> MIEKLIHFINNDLLEGAADDLDQNTPLLELGILDSLSMVLLLAHIDQQYGVKIPEHEINPEHFENVATLAALINQLS;> MNFEWTHEQAELFEHALRFGKELSAPLQEDNGFPRDNWNALGDFGYFGLPIPEKYAKDGSGFDILTTIKIIEGLGQSCTDTGLLFAGAAHTFACSMPILEHGSETLKHQLLPDLATGRKIAANAISEASAGSDISNLATTAQKEGDYYVLNGGKSYVTNGSIADYYVVYATTNKKHGYLGQTAFVVPRNTPGISVGNDYHKLGLRSAPLNQVFFDNCTIHKDYALGREGQGARIFAASMDWERCCLFAIFVGAMQRDLNQCIEYANTRMQGDKTISRFQAVSHRIADMGVRLESARLMLYYAAWQKSQDVDNTKAVAMSKLAISEAFVQSGIDSIRVHGALGYLDEGRVNNSIKDALGSVL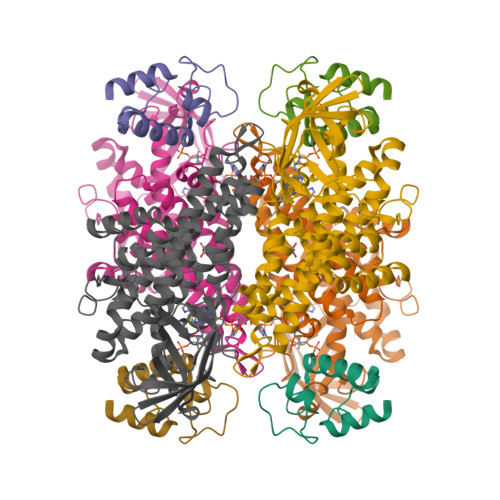FSGTSDIQRELICNRLGLL(25S)-3-oxocholest-4-en-26-oyl-CoA | C48 H76 N7 O18 P3 S | 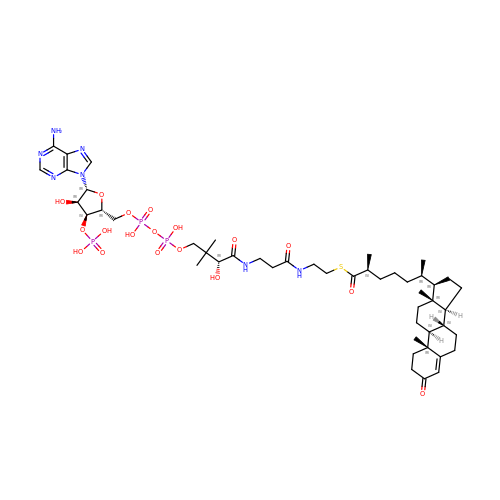QHTNQHCVKNUPEI-ZAXAEIALSA-N6-(cyclopentylamino)pyridine-3-carboxamide 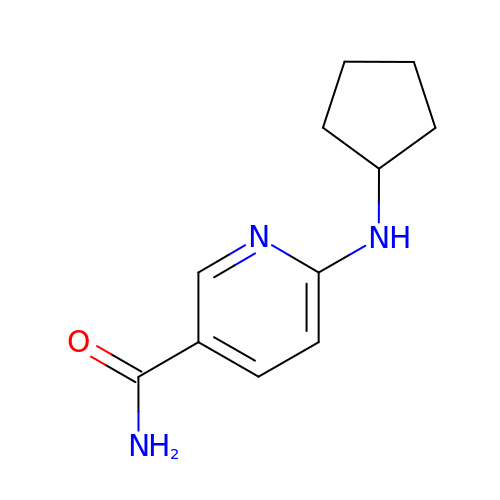| C11 H15 N3 O | HTKJVDABQHUEPR-UHFFFAOYSA-N>GPGYQMDIPKFKRLPRHIAIIPDGNRRWALARGLEKHEGYSSGIIPGLEVYDICVKIGIGEVTFFGFTQDNTKRPQIQRKAFTDACIKSVQEIAKRDAEILVVGNTNSDIFPEELLEYTKRTKVGKGKIKINFLINYGWYWDLTYAYDNSPDGKKMIENIASAEIPRVDLLIRWGGRCRLS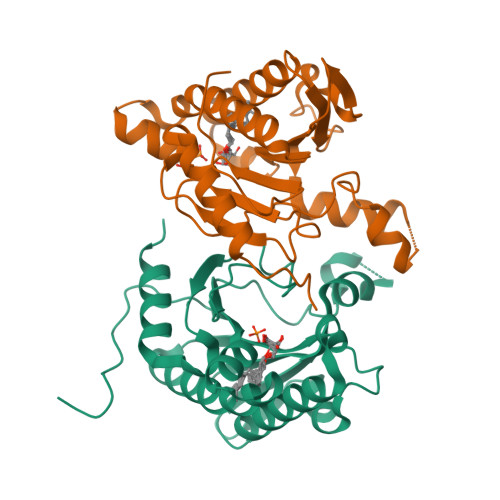GMLPVQTVYSDIYVVDEMWPDFKPEHLFKALEFYQNQDITLGG[8x]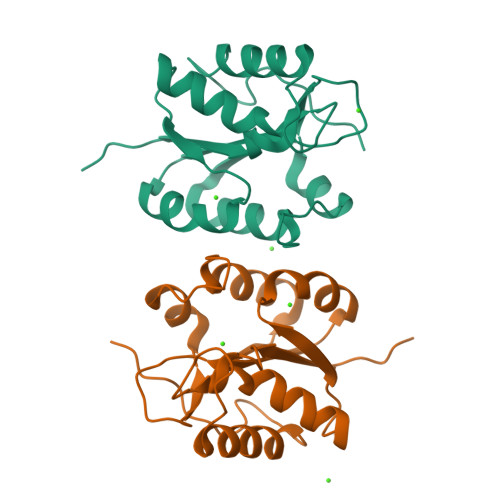>[2x]ASAVTDVLLCVGNSMMGDDGAGPLLAEKCAAAPKGNWVVIDGGSAPENDIVAIRELRPTRLLIVDATDMGLNPGEIRIIDPDDIAEMFMMTTHNMPLNYLIDQLKEDIGEVIFLGIQPDIVGFYYPMTQPIKDAVETVYQRLEGWEGNGGFAQLAVEEE> MAKPKDPIYVWAAADVNLPGTGRPNKSKPIDDLLAKGYDKGQKPAAEEFNYILNMSSAWVNWIVNEKFPELEAEIARLLAELENRINQQLAVIRQDIAQLRQDVADLRRYVDQKVQELKQEIQGVRNDLNKLRQDFDAAITQVNGRIDDLEPRLVPIG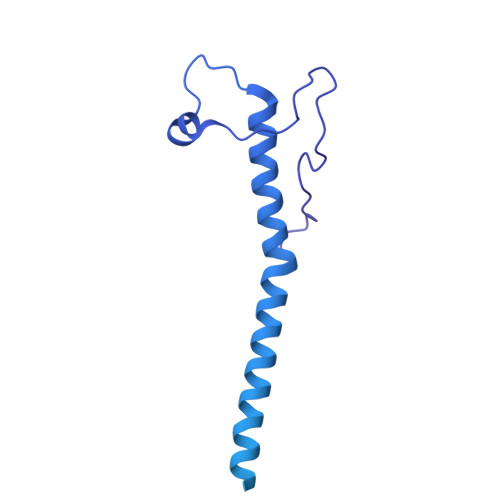AVIPWPGATVPDGWLECSGQVFNTGQNPKLYSVLGRNVVPDYRGLFLRGWAHGSDANDPDAGRALGSVQGDAIRNITGYFPADIGNSNFIGRYVGGAFRDDGSLTSGDDGTRSNEVRKYSFDASREVPVAAENRPKNIAVMYIIKTDQAQSSGGNSPTAIVVSPDTITNRIGYAVKATASVLPASISGQYPISWSTQNAAVATVDGSGNISLVGPGETNIIASISTGMNVVIRVTSYSVLTSISIADPGQITVTESKMLVVTKSPSSANEPLQFLSNNSGVAAVNDAGYVIGVSAGSATITVRGTLSGVSSTRAVTIIPEQVEESVQDNRLGAVGSYIPPSPSSNVMSWTFQAPQGCALTGIIVQENESNSGDNIGGVYYKPIQKKVNGVWVTITG>IVGGTASVRGEWPWQVTLHTTSPTQRHLCGGSIIGNQWILTAAHCFYGVESPKILRVYSGILQQSEIKEDTSFFGVQEIIIHDQYKMAESGYDIALLKLETTVQYTDSQRPISLPSKGDRNVIYTDCWVTGWGYRKLRDKIQNTLQKAKIPLVTNEECQKRYRGHKITHKMICAGYRE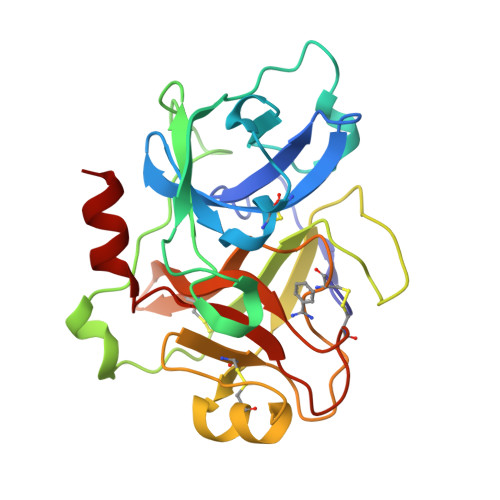GGKDACKGDSGGPLSCKHNEVWHLVGITSWGEGCAQRERPGVYTNVVEYVDWILEKTQ[4x]3-{2,6,8-TRIOXO-9-[(2R,3S,4R)-2,3,4,5-TETRAHYDROXYPENTYL]-1,2,3,6,8,9-HEXAHYDRO-7H-PURIN-7-YL}PROPYL DIHYDROGEN PHOSPHATE | C13 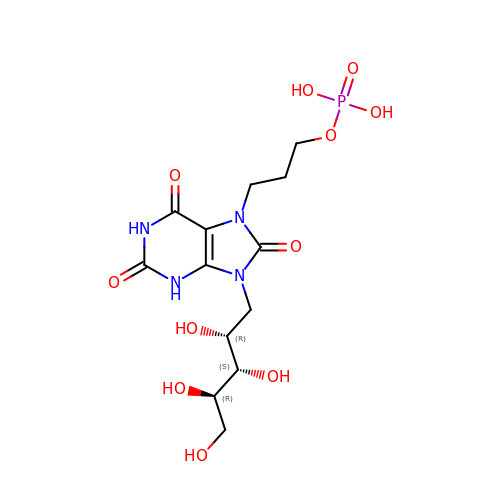H21 N4 O11 P | KPHFGOGGKPGLTM-BHNWBGBOSA-N1-palmitoyl-2-oleoyl-sn-glycero-3-phosphoglycerol 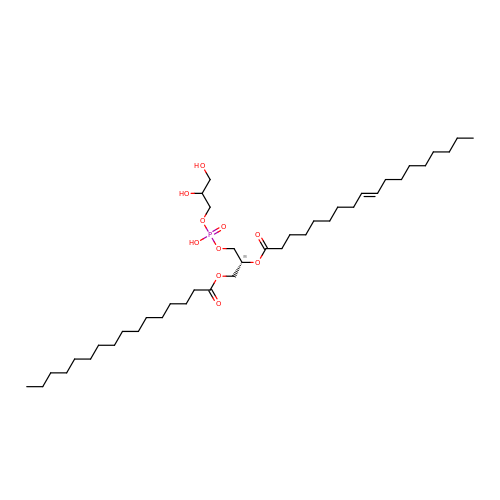| C40 H77 O10 P | PAZGBAOHGQRCBP-YWIOZPJLSA-N> SEFSRHSEKIAIRDFQVGDLVLIILDERHDNYVLFTVSPTLYFLHSESLPALDLKPGEGASGASRRPWVLGKVMEK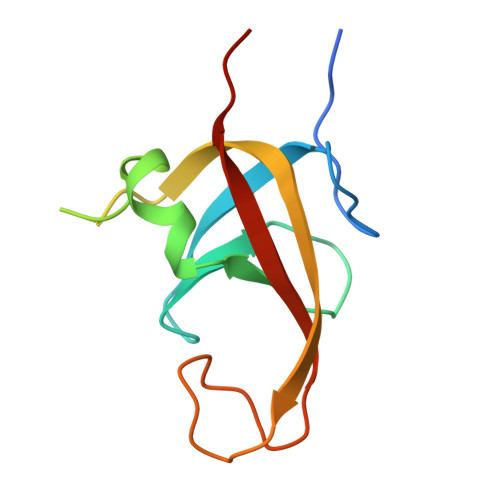EYCQAKKAQNRFKVPLGTKFYRVKAVSWNKKV>MPMFTVNTNVPRASVPEGLLSELTQQLAQATGKPAQYIAVHVVPDQLMTFSGSSDPCALCSLHSIGKIGGAQNRTYSKLLCGLLADRLHISPDRIYINYYDMSAANVGWNGSTFALEHHHHHH[3x]

Macrophage migration inhibitory factor (MIF) is a pro-inflammatory cytokine with pleiotropic functions in various pathophysiological processes. Unlike all other cytokines, MIF has a tautomerase activity, and it performs this enzymatic function through an N-terminal catalytic proline base. Our analysis showed that like human MIF, MaMIF also forms a trimer in solution. Alignment of the primary sequences of MIF from hamster, mouse, and human was performed with PRALINE program. Figure 2A indicates that MaMIF shares 93% and 89% sequence identity with mouse MIF and human MIF, respectively.

The crystal structure of MaMIF was resolved to 1.8 Å resolution. It forms a trimer, with three identical molecules in an asymmetric unit. A monomer of MaMIF is made up of six beta strands, four of which form a mixed beta sheet within one subunit, two antiparallel alpha helices and two shorter beta strands on either end of the sheet. The trimer adopts a barrel-like architecture formed by three inter-connected monomeric subunits, as has been reported for other MIF structures. The trimeric MaMIF structure is retained by the short beta strands β3 of one monomer and β6 of the third monomer becoming part of the beta sheet formed by the beta strands β1, β2, β4 and β5 of the second monomer in between, together forming a six-stranded beta sheet. Herein, β3 of monomer-1 comes in close proximity and form hydrogen-bond network, typical of beta sheets, with β2 of the monomer-2 and β6 of monomer-3 comes close to β5 of monomer-2. This contribution of beta strands by all three monomers to their respective adjacent monomers to form beta sheets seems to provide stability to the trimeric structure. The alignment reveals that the residues responsible for tautomerase activity and substrate binding such as Pro2, Lys33, Ile65, Tyr96, and Asn98 are conserved in MaMIF as well. As the residues of the catalytic pocket and ISO-1 binding are completely conserved in MaMIF, ISO-1 and other similar compounds binding to the catalytic pocket would block MaMIF catalytic function as well. However, the MaMIF structure from this work did not have any sulfate ions, presumably because the final crystallization condition did not have any sulfate.> AMDHVEFGLTYSQLMTLKDAMLQLDPNAKTWMDIEGRPEDPVEIALYQPSSGCYIHFFREPTDLKQFKQDAKYSHGIDVTDLFATQPGLTSA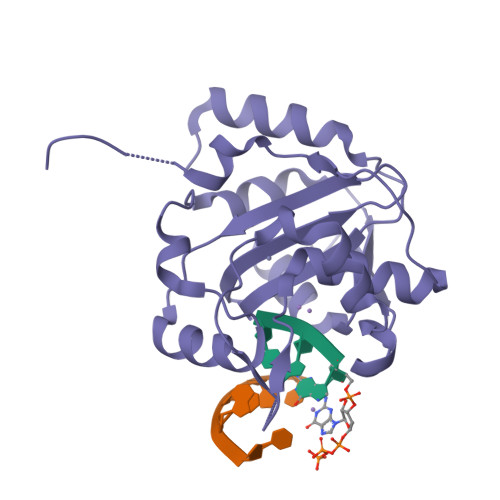VIDALPRNMVITCQGSDDIRKLLESQGRKDIKLIDIALSKTDSRKYENAVWDQYKDLCHMHTGVVVEKKKRGGKEEITPHCALMDCIMFDAAVSGGLNTSVLRAVLPRDMVFRTSTPRVVL>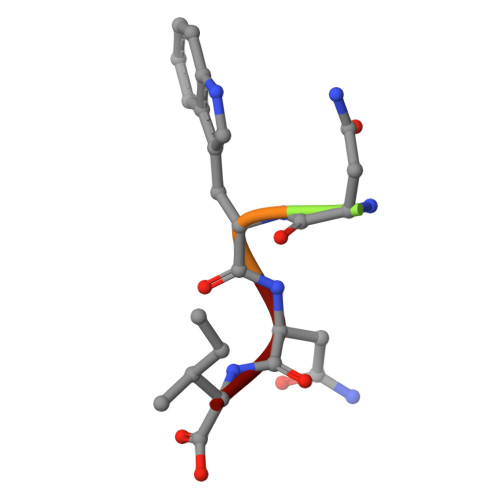 MNWNI> MLRREFGPKYTAKINEAEENWQARAEAIKKGKKQNTWDLFEERGYVKDTAGTKEHIAELMRTRRIGAYVGIDPTAPSLHVGHLLPLMPLFWMYLEGYKAFTLIGGSTAKIGDPTGRLKSRDHLSSSDATMNMTKIHYQLKKLWENVDTQMRARGYEADWARKRGIVNNNHWWNKQPMLEVLRR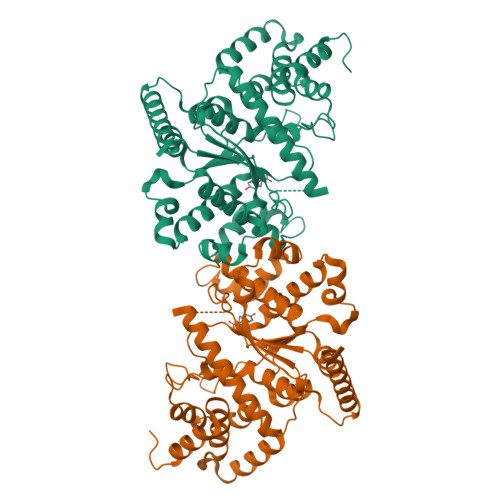VGHALRIGPMLSRDTVKNKMTQGDGVSFAEFTYPIMQGWDWFELFYQQGVQMQIGGSDQYGNIISGLEVVKAARESEPDPQERKYVTPKTALDECVGFTVPLLTDSSGAKFGKSAGNAIWLDPYQTSVFDFYGYFVRRSDQEVENLLKLFTFMPISEITKTMEEHIKDPSKRVAQHTLAREVVTLVHGKQEASAAEDQHRMMYTGQMTI Here, we report sub-particle cryoEM reconstructions of HCMV virions at 2.9 Å resolution revealing structures resembling non-coding transfer RNAs (tRNAs) associated with the virion’s capsid-bound tegument protein, pp150. Through deep sequencing, we show that these RNA sequences match human tRNAs, and we built atomic models using the most abundant tRNA species. Based on our models, tRNA recruitment is mediated by the electrostatic interactions between tRNA phosphate groups and the helix-loop-helix motif of HCMV pp150. The DNA confining hexon channel is “secured” from the outside by β-herpesvirus-specific tegument protein pp150, whose N-terminal one-third (pp150nt) is resolved.

Each L-shaped density interacts with three pp150 subunits atop a triplex: one at the corner of the L, and one at each of the two arms of the L. Each arm of the L-shaped density has a 2.3 nm width and has coaxial double helices, which are the defining feature of nucleic acid. Using the sequence of the most abundant tRNA species, we built atomic models into the tRNA density. The atomic model consists of four leaflets—acceptor stem (1–8 and 65–71 nt), D-arm (9–26 nt), anticodon arm (27–43 nt), and T-arm (48–64 nt). One tRNA bridges over three pp150 molecules, two of which interact with each other (pp150nt-a and pp150nt-b) while the third is slightly farther apart (pp150nt-c). Four interaction sites between tRNA and pp150s can be identified, all of which might be mediated by electrostatic interactions with the phosphate groups. Among the three, pp150nt-a has the most extensive interactions with the tRNA, binding to both the T-arm (at 25 Gln, 26 Lys and 34 His, 39 Lys, and 40 Lys) and the loop of the D-arm (9 Gln and 11 Arg). pp150nt-b interacts with the phosphate groups in the base-stacked region of the anticodon arm (at 22 His, 26 Lys, and 36 Lys). These interactions only involve the phosphate groups, which introduce less selectivity than base-stacked groups during the recruitment of tRNA, indicating that pp150 could bind to different types of tRNA as shown by the sequencing data. At the two ends of the L-shaped structure, the anticodon and the CCA tail are also located in proximity to pp150, contacting the highly positively charged regions of pp150nt-b and pp150nt-c, respectively. We found that cryoEM densities of tRNAs on the Tb, Td, and Te have the highest resolution, whereas the tRNA on Ta has a much weaker density, not observable at a higher threshold. The set-of-three pp150 proteins on Tb, Td, and Te match well, and above those triplexes are the highest density of tRNA.

>MSLQFIGLQRRDVVALVNFLRHLTQKPDVDLEAHPKILKKCGEKRLHRRTVLFNELMLWLGYYRELRFHNPDLSSVLEEFEVRCVAVARRGYTYPFGDRGKARDHLAVLDRTEFDTDVRHDAEIVERALVSAVILAKMSVRETLVTAIGQTEPIAFVHLKDTEVQRIEENLEGVRRNMFCVKPLDLNLDRHANTALVNAVNKLVYTGRLIMNVRRSWEELERKCLARIQERCKLLVKELRMCLSFDSNYCRNILKHAVENGDSADTLLELLIEDFDIYVDSFPQS[9x]>[2x]VTDSINWASGEDDHVVARAEYDF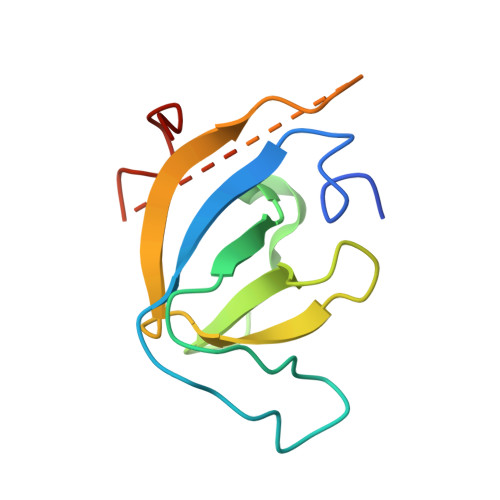AAVSEEEISFRAGDMLNLALKEQQPKVRGWLLASLDGQTTGLIPANYVKILGKRKGRKTVESSGGGGSTATDRWYDEYHPEE> V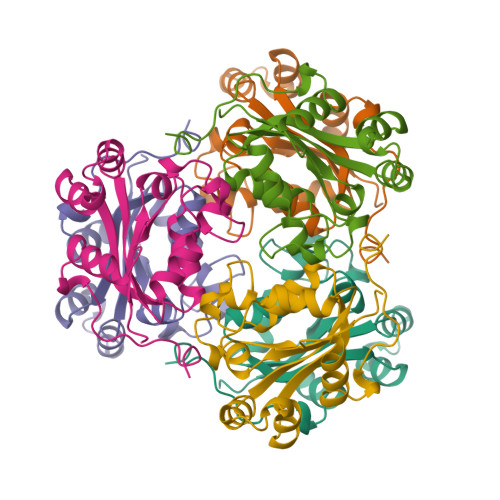NKERTFLAVKPDGVARGLVGEIIARYEKKGFVLVGLKQLVPTKDLAESHYAEHKERPFFGGLVSFITSGPVVAMVFEGKGVVASARLMIGVTNPLASAGGSIRGDFGVDVGRNIIHGSDSVESANREIALWFKPEELLTEVKPNPNLYE>[2x]SMDDDQVAFSFILDNIVTQKMMAVPDSWPFHHPVNKKFVPDYYKVIVNPMDLETIRKNI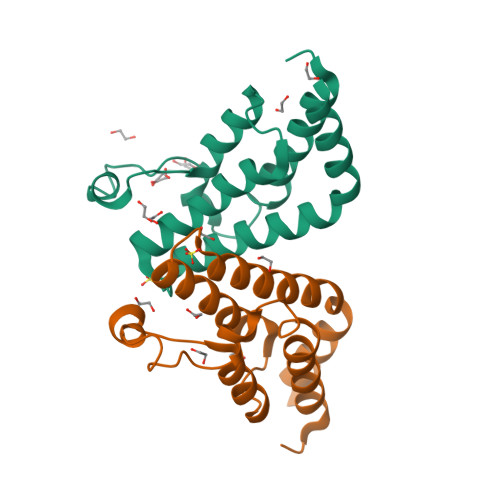SKHKYQSRESFLDDVNLILANSVKYNGPESQYTKTAQEIVNVCYQTLTEYDEHLTQLEKDICTAKEAALEEAELESLD>[2x]MMGDL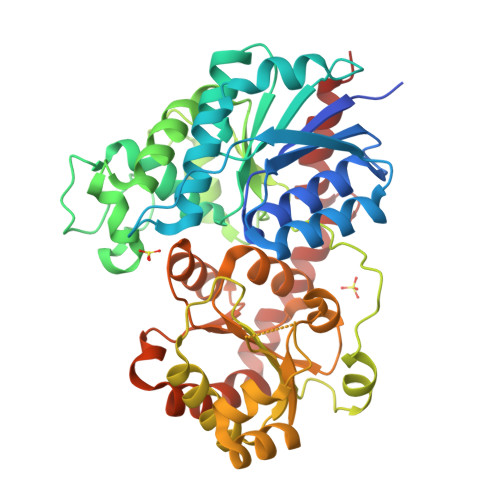TTSFPATTLTTNDQPHVVVCSGAGMGHLTPFLNLASALSSAPYNCKVTLLIVIPLITDAESHHISSFFSSHPTIHRLDFHVNLPAPKPNVDPFFLRYKSISDSAHRLPVHLSALSPPISAVFSDFLFTQGLNTTLPHLPNYTFTTTSARFFTLMSYVPHLAKSSSSSPVEIPGLEPFPTDNIPPPFFNPEHIFTSFTISNAKYFSLSKGILVNTFDSFEPETLSALNSGDTLSDLPPVIPIGPLNELEHNKQEELLPWLDQQPEKSVLYVSFGNRTAMSSDQILELGMGLERSDCRFIWVVKTSKIDKDDKSELRKLFGEELYLKLSEKGKLVKWVNQTEILGHTAVGGFLSHCGWNSVMEAARRGVPILAWPQHGDQRENAWVVEKAGLGVWEREWASGIQAAIVEKVKMIMGNNDLRKSAMKVGEEAKRACDVGGSSATALMNIIGSLKR>GSHNATSGHEDMPVERILEAELAVEPKTESYGDMNMENSTNDPVTNICHAADKQLFTLVEWAKRIPHFSDLTLEDQVILLRAGWNELLIASFSHRSVSVQDGILLATGLHVHRSSAHSAGVGSIFDRVLTELVSKMKDMQMDKSELGCLRAIVLFNPDAKGLSNPSEVETLREKVYATLEAYTKQKYPEQPGRFAKLLLRLPALRSIGLKCLEHLFFFKLIGDTP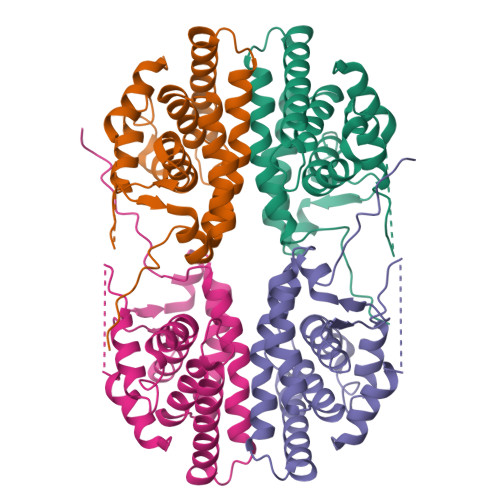IDTFLMEMLETPLQIT[4x]>GPDSMGAAAAEADRTLFVGNLETKVTEELLFELFHQAGPVIKVKIPKDKDGKPKQFAFVNFKHEVSVPYAMNLLNGIKLYGRPIKIQFRS[7x];>GPDSMRFKPGVISEELQDALGVTDKSLPPFIYRMRQLGYPPGWLK[7x]

In the nucleoplasm, however, hMTR4 binds the RBM7 and ZCCHC8 proteins, forming the metazoan-specific nuclear exosome targeting (NEXT) complex27. NEXT promotes the exosomal degradation of non-coding promoter-upstream transcripts, enhancer RNAs28 and 3′-extended products of histone- and small nuclear RNA transcription. We conclude that ZCCHC8 is a scaffolding subunit that bridges the interaction between RBM7 and hMTR4. In this work, we have shown that RBM7RRM binds a proline-rich segment of ZCCHC8 at the back helical surface and is able to concomitantly bind RNA.

From the pull-down assays with the corresponding protein constructs (lane 6), we could demonstrate that ZCCHC8285–324 (encompassing the proline-rich region downstream of the Zinc-knuckle domain, ZCCHC8Pro) is sufficient to bind RBM71–86 (spanning the RRM domain, RBM7RRM). The complex between ZCCHC8Pro and RBM7RRM yielded crystals diffracting to about 2.85 Å resolution, with seven complexes in the asymmetric unit. To obtain experimental phases, we co-crystallized the complex in the presence of heavy-atom compounds. Co-crystallization with Samarium chloride yielded a different crystal form diffracting to 2.0 Å resolution and containing a single copy of the complex in the asymmetric unit. The coordinates of the Sm-derivatized RBM7RRM–ZCCHC8Pro complex allowed solving the structure of the native complex (Rfree of 30.0% and R-factor of 26.2%). As the two structures are very similar, we focused on the highest-resolution atomic model, which includes residues 286–324 of ZCCH8 and residues 7–86 of RBM7.>MAGVLPAHGTQHGIRLPLRSGLGGAPLGLRLPRETDEEPEEPGRRGSFVEMVDNLRGKSGQGYYVEMTVGSPPQTLNILVDTGSSNFAVGAAPHPFLHRYYQRQLSSTYRDLRKGVYVPYTQGK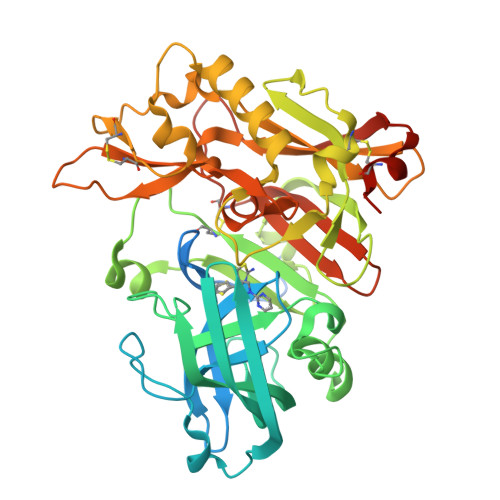WEGELGTDLVSIPHGPNVTVRANIAAITESDKFFINGSNWEGILGLAYAEIARPDDSLEPFFDSLVKQTHVPNLFSLQLCGAGFPLNQSEVLASVGGSMIIGGIDHSLYTGSLWYTPIRREWYYEVIIVRVEINGQDLKMDCKEYNYDKSIVDSGTTNLRLPKKVFEAAVKSIKAASSTEKFPDGFWLGEQLVCWQAGTTPWNIFPVISLYLMGEVTNQSFRITILPQQYLRPVEDVATSQDDCYKFAISQSSTGTVMGAVIMEGFYVVFDRARKRIGFAVSACHVHDEFRTAAVEGPFVTLDMEDCGYNIPQTDEST[2x]>[7x]MAEQKSSNGGGGGGDVVINVPVEE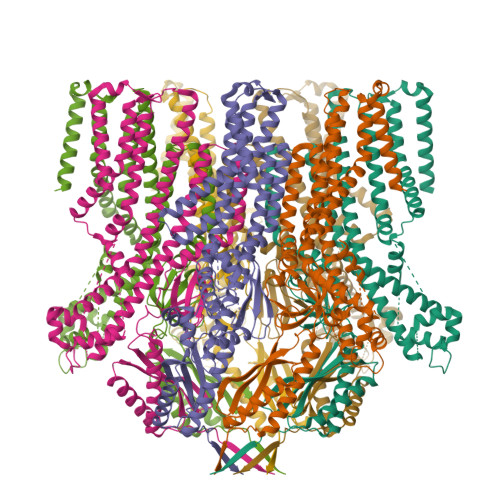ASRRSKEMASPESEKGVPFSKSPSPEISKLVGSPNKPPRAPNQNNVGLTQRKSFARSVYSKPKSRFVDPSCPVDTSILEEEVREQLGAGFSFSRASPNNKSNRSVGSPAPVTPSKVVVEKDEDEEIYKKVKLNREMRSKISTLALIESAFFVVILSALVASLTINVLKHHTFWGLEVWKWCVLVMVIFSGMLVTNWFMRLIVFLIETNFLLRRKVLYFVHGLKKSVQVFIWLCLILVAWILLFNHDVKRSPAATKVLKCITRTLISILTGAFFWLVKTLLLKILAANFNVNNFFDRIQDSVFHQYVLQTLSGLPLMEEAERVGREPSTGHLSFATVVKKGTVKEKKVIDMGKVHKMKREKVSAWTMRVLMEAVRTSGLSTISDTLDETAYGEGKEQADREITSEMEALAAAYHVFRNVAQPFFNYIEEEDLLRFMIKEEVDLVFPLFDGAAETGRITRKAFTEWVVKVYTSRRALAHSLNDTKTAVKQLNKLVTAILMVVTVVIWLLLLEVATTKVLLFFSTQLVALAFIIVSTCKNLFESIVFVFVMHPYDVGDRCVVDGVAMLVEEMNLLTTVFLKLNNEKVYYPNAVLATKPISNYFRSPNMGETVEFSISFSTPVSKIAHLKERIAEYLEQNPQHWAPVHSVVVKEIENMNKLKMALYSDHTITFQENRERNLRRTELSLAIKRMLEDLHIDYTLLPQDINLTKKNSLEVLFQ>MSPTAKPNSQVSLNQESVLRRITARIRQSLELEDIITATTAEVRALLGTDRVMIYKFHPDGSGQVIAESIYENRLPSLLGLNFPADDIPPQARELLVKSKVRSIVDVATGMIGQSPVHDLETGELISEDICYRPVDSCHVEYLTAMGVKSSVVAPI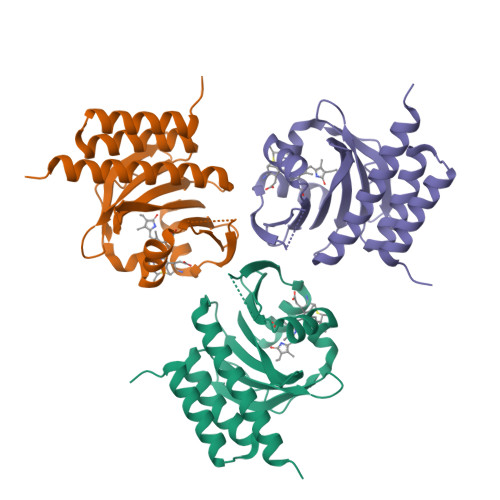FCQDELWGLLVSHHSENRTVSEDELEAMQMIVDQLAVAIAQSHLEHHHHHH[3x]>MARIAQHISELIGGTPLVRLNSVVPDGAGTVAAKVEYLNPGGSSKDRIAVKMIEAAEASGQLKPGGTIVEPTSGNTGVGLALVAQRRGYKCVFVCPDKVSEDKRNVLIAYGAEVVVCPTAVPPHDPASYYSVSDRLVRDIDGAWKPDQYANPEGPASHYVTTGPEIWADTEGKVTHFVAGIGTGGTITGAGRYLKEVSGGRVRIVGADPEGSVYSGGAGRPYLVEGVGEDFWPAAYDPSVPDEIIAVSDSDSFDMTRRLAREEAMLVGGSCGMAVVAALKVAEEAGPDALIVVLLPDGGRGYMSKIFNDAWMSSYGFLRSRLDGSTEQSTVG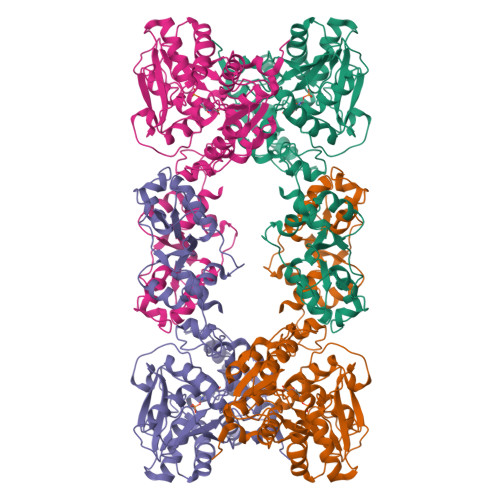DVLRRKSGALPALVHTHPSETVRDAIGILREYGVSQMPVVGAEPPVMAGEVAGSVSERELLSAVFEGRAKLADAVSAHMSPPLRMIGAGELVSAAGKALRDWDALMVVEEGKPVGVITRYDLLGFLSEGAGRRKLAAALEHHHHHH[4x]>MNDPVLLNLPMNVTISENSPVSSFVAHVLASDADSGCNALLTFNITAGNRERAFFINATTGIVTVNRPLDRERIPEYRLTVSVKDNPENPRIARKDFDLLLVSLADENDNHPLFTEGTYQAEVMENSPAGTPLTVLNGPILALDADEDVYAVVTYQLLGTHSDLFVIDNSTGVVTVRSGIIIDREAFSPPFLELLLLAEDIGQLNGTAHLFIT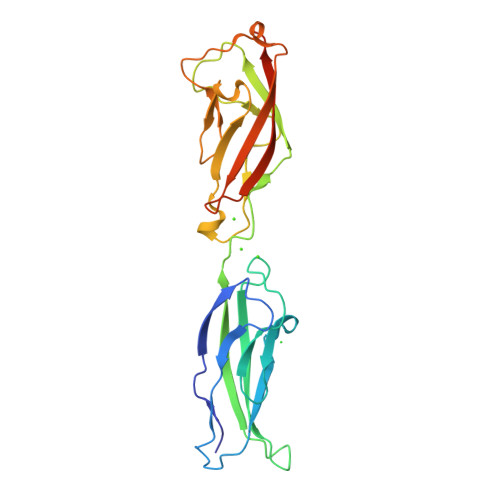ILDDNLEHHHHHH[2x]>MKLPVREFDAVVIGAGGAGMRAALQISQSGQTCALLSKVFPTRSHTVSAQGGITVALGNTHEDNWEWHMY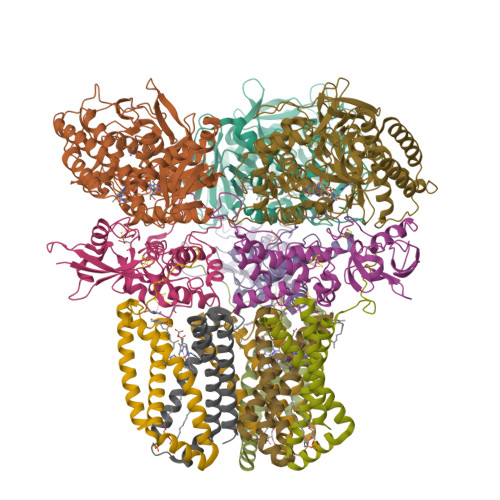DTVKGSDYIGDQDAIEYMCKTGPEAILELEHMGLPFSRLDDGRIYQRPFGGQSKNFGGEQAARTAAAADRTGHALLHTLYQQNLKNHTTIFSEWYALDLVKNQDGAVVGCTALCIETGEVVYFKARATVLATGGAGRIYQSTTNAHINTGDGVGMAIRAGVPVQDMEMWQFHPTGIAGAGVLVTEGCRGEGGYLLNKHGERFMERYAPNAKDLAGRDVVARSIMIEIREGRGCDGPWGPHAKLKLDHLGKEVLESRLPGILELSRTFAHVDPVKEPIPVIPTCHYMMGGIPTKVTGQALTVNEKGEDVVVPGLFAVGEIACVSVHGANRLGGNSLLDLVVFGRAAGLHLQESIAEQGALRDASESDVEASLDRLNRWNNNRNGEDPVAIRKALQECMQHNFSVFREGDAMAKGLEQLKVIRERLKNARLDDTSSEFNTQRVECLELDNLMETAYATAVSANFRTESRGAHSRFDFPDRDDENWLCHSLYLPESESMTRRSVNMEPKLRPAFPPKIRTY[3x];>MRLEFSIYRYNPDVDDAPRMQDYTLEADEGRDMMLLDALIQLKEKDPSLSFRRSCREGVCGSDGLNMNGKNGLACITPISALNQPGKKIVIRPLPGLPVIRDLVVDMGQFYAQYEKIKPYLLNNGQNPPAREHLQMPEQREKLDGLYECILCACCSTSCPSFWWNPDKFIGPAGLLAAYRFLIDSRDTETDSRLDGLSDAFSVFRCHSIMNCVSVCPKGLNPTRAIGHIKSMLLQRNA[3x];>MIRNVKKQRPVNLDLQTIRFPITAIASILHRVSGVITFVAVGILLWLLGTSLSSPEGFEQASAIMGSFFVKFIMWGILTALAYHVVVGIRHMMMDFGYLEETFEAGKRSAKISFVITVVLSLLAGVLVW[3x];>[3x]MVSNASALGRNGVHDFILVRATAIVLTLYIIYMVGFFATSGELTYEVWIGFFASAFTKVFTLLALFSILIHAWIGMWQVLTDYVKPLALRLMLQLVIVVALVVYVIYGFVVVWGV3-phenyl-1~{H}-pyrrolo[3,4-g]indol-8-one 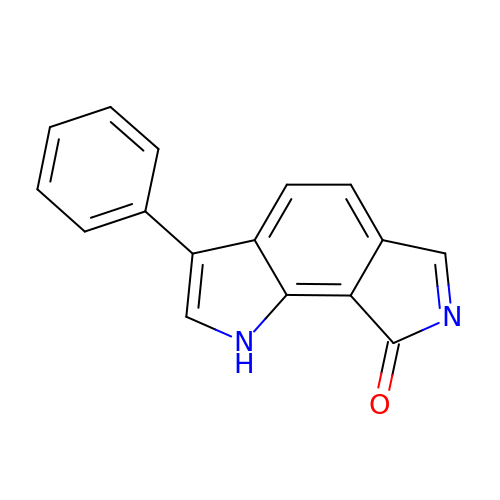| C16 H10 N2 O | YJGNZVVUIPDSRL-UHFFFAOYSA-N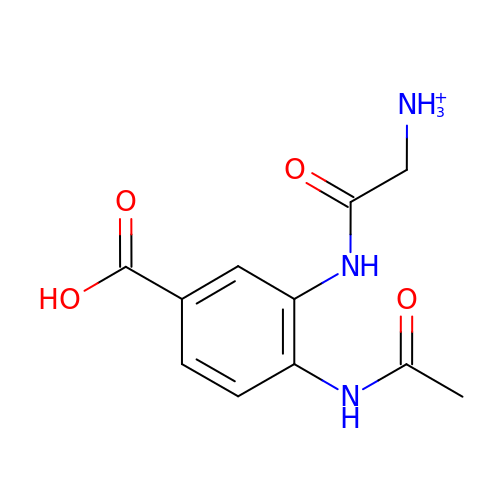4-(ACETYLAMINO)-3-[(AMINOACETYL)AMINO]BENZOIC ACID | C11 H14 N3 O4 | FJGXEWVOOHZQDN-UHFFFAOYSA-O> MNAVEIQGVSQRYGSMTVLHDLNLNLGEGEVLGLFGHNGAGKTTSMKLILGLLSPSEGQVKVLGRAPNDPQVRRQLGYLPENVTFYPQLSGRETLRHFARLKGAALTQVDELLEQVGLAHAADRRVKTYSKGMRQRLG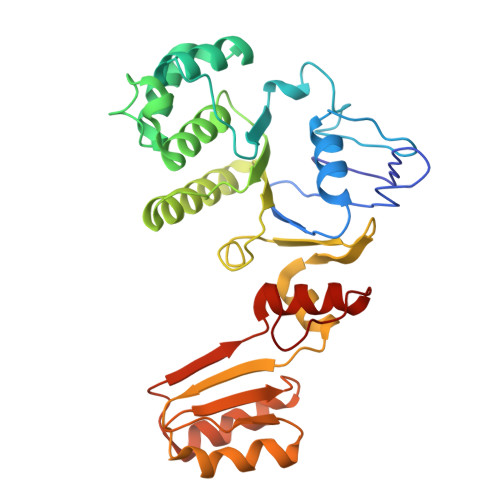LAQALLGEPRLLLLDEPTVGLDPIATQDLYLLIDRLRQRGTSIILCSHVLPGVEAHINRAAILAKGCLQAVGSLSQLRAEAGLPVRIRASGISERDSWLQRWTDAGHSARGLSESSIEVVAVNGHKLVLLRQLLGEGEPEDIEIHQPSLEDLYRYYMERAGDVRAQEGRL>[40x]GGTDPATMVNNICTFILGPFGQS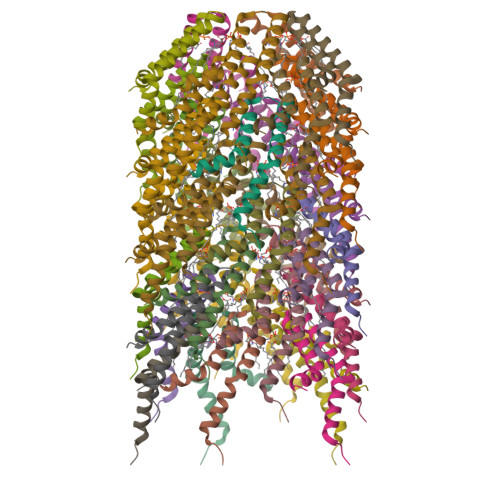LAVLGIVAIGISWMFGRASLGLVAGVVGGIVIMFGASFLGKTLTGG>GGRMQLTADQVEKYKSDGYVLLEGAFSPEEVHVMRQALKKDQEVQGPHRILEEDGRTVRALYASHTRQSVFDQLSRS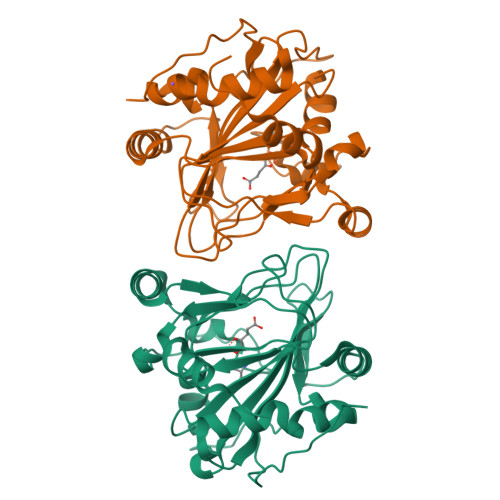DRLLGPATQLLECDLYIHQFKINTKRAFGGDSWAWHQDFIVWRDTDGLPAPRAVNVGVFLSDVTEFNGPVVFLSGSHQRGTVERKARETSRSDQHVDPDDYSMTPAELSQMVEKHPMVSPKAASGSVMLFHPEIIHGSAPNISPFARDLLIITYNDVANAPKPAGEPRPEYVIGRDTTPLVSRSGPLHEAA[2x]>GSGGGMFGAFVSHRLWSDSGCTTTCITNSIANYVAFGEQIGFPFKSAQVFIAGPRKAVINIQEDDKVELLKMIVKHNLWVVAHGTYLDVPWSRRSAFVTHFIQQELLICKEVGIKGLVLHLGAVEPELIVEGLKKIKPVEGVVIYLETPHNKHHTYKYSTMEQIKELFLRIRNTRLKQIGLCIDTAHIWSSGVNISSYNDAGQWLRSLENIHSVIPPSHIMFHLNDAATECGSGIDRHASLFEGMIWKSYSHKIKQSGLYCFVEYITRHQCPAILERNLGSSMQLQTALTAEFTTLKSLLK[2x]

ASFV AP endonuclease (AsfvAP) catalyzes DNA cleavage reaction at the abasic site and is a key enzyme of ASFV base excision repair (BER) system. AsfvAP belongs to the class II AP endonuclease family; it mainly catalyzes DNA cleavage reaction at the 5′ side of abasic site (AP), generating 3′-OH group and 5′-deoxyribose phosphate (dRP). AsfvAP is of α/β fold in nature; the β-strands form one β-barrel in the center, surrounded by α-helices at the outer side. AsfvAP possesses many unique structural features, including one narrower nucleotide-binding pocket at the active site, the C16–C20 disulfide bond-containing region, and histidine-rich loop.

AsfvAP/DNA-1 crystal belongs to P21 space group. Per asymmetric unit contains two AsfvAP/DNA-1 complexes, and each complex is formed by one AsfvAP protein and one DNA-1 molecule. However, as confirmed by the clear 2Fo–Fc electron density maps, the DNA was cleaved at the 5′ side of the abasic site in the structure. Three well-defined Zn2+ ions were captured in the structure, coordinating with the side chains of His78, His115, Glu142, Asp179, His182, Asp231, His233, and Glu271. In addition, the Zn2+ ions also forms direct coordination with the 5′-phosphate group of dRP, the product of the abasic site cleavage. Taken together, these observations demonstrated the catalytic activity of AsfvAP and indicated that the AsfvAP/DNA-1 complex was assembled in a catalytic form. The AsfvAP/DNA-1 complex structure was refined at atomic resolution (2.35 Å), which revealed the detailed basis for target DNA recognition by AsfvAP. The DNA molecule mainly interacts with AsfvAP in three regions: R1, R2, and R3. As revealed by our AsfvAP/DNA-1 complex, the S-S bond was formed between Cys16 and Cys20 within the R1 region.In this study, we identified four enzymes (two GH183 endo-d-arabinanases, GH172 exo-α-d-arabinofuranosidase, and GH116 exo-β-d-arabinofuranosidase) from Microbacterium arabinogalactanolyticum. These enzymes completely degraded the complex d-arabinan core structure of lipoarabinomannan and arabinogalactan in a concerted manner. Furthermore, through biochemical characterization using synthetic substrates and X-ray crystallography, we elucidated the mechanisms of substrate recognition and anomer-retaining hydrolysis for the α- and β-d-arabinofuranosidic bonds in both endo- and exo-mode reactions. We propose a d-arabinan-degrading pathway for Mi. arabinogalactanolyticum based on its gene cluster and four characterized enzymes.

A complex-form crystal was prepared using a catalytic residue mutant (D51N) for the co-crystallization of A9LT. In the catalytic domain, the active site on the front side of a 5-bladed β-propeller fold contained a linear tetrasaccharide with an acetonide tag (A4LT). Unexpectedly, a linear tetrasaccharide without the tag (A4L) bound to a putative carbohydrate-binding module (CBM) domain that adopted a β-sandwich fold was revealed. The bound A4LT molecule in the complex crystal form spans subsites −3 to +1, and the arabinofuranose ring at subsite −1 adopts a 3E conformation to hold the α-anomeric scissile bond in the pseudoaxial position. The side-chain oxygen of Asp33 is located 2.8 Å from the anomeric C1 atom, making it suitable for in-line nucleophilic attack. Asn51(Asp) forms a hydrogen bond with the glycosidic bond oxygen between subsites −1 and +1, suggesting that it is the catalytic acid/base residue. Pro141, Arg198, and Leu292 form hydrogen bonds with A4LT, while Tyr293 and Trp138 form stacking interactions above and below the cleft. Glu243 is the third Asp/Glu residue in the active site cleft and supports the side chain position of Arg198, which plays a pivotal role in holding sugars at subsites −3 and −2. The activity of the D33N, D51N, E243A, and E243Q mutants toward A22BβT was nearly abolished, confirming that all three Asp/Glu residues are catalytically essential. The arabinose unit at subsite A is sandwiched between the aromatic side chains of Phe379 and Trp468, and hydrogen bonds from Asp365, Arg381, and Gln470 are formed.

>[4x]MTTSRTPATVVEKLTGPDAPNNTWGRWDIKATDLGIMWDDGAGHVLTAFGNTFGNSWTGPGGGAPPNGNWRSNVLVRSSDGDLADGMLFDWAAQGPQGVAREIIPSKKINGVEITTIPTTGISVGKRQYLGFMSVKQWGPPGVWDTNFAGIAYSDDGGGTWKVSDTRWENADGHDPFQMQAWVQKGGTIYVFGTQNGRNGPASVAKVPASKLLDKSAFRYWNGTDWSRKESDAVPVMDAPMSEMSVQYDAYSKRFLMMTLSGEDIIMRTATAPEGPWTPAQTVASSTDYPALYGGYFHPWNKDGEIYFTMSQWNPYNVYLMRLRIDRDGNIIDPNLVTDASFERSTTLGDGTNGTWAAKPNSGIDNAPAAGFTGDHRAFVRYNSGWRDIWQDVAVERGAKYRLTGFLRTSVNSDNGFFGARTLDGVPIGEINFHSVGAWTRFTVEFDAGDRDAVQVFGGVWTNSGDIWMQLDDVSLTKVRLEHHHHHH Carboxyl esterases (EC 3.1.1.1) and lipases (EC 3.1.1.3) are enzymes that catalyze the cleavage of an ester bond between a carboxylic acid and an alcohol group. The TtEst2 enzyme reveals an open substrate binding site, which is solvent accessible due to the absence of the usual ‘cap’ domain which is present in TtEst.

The purified TtEst2 enzyme has been crystallized and the structures have been determined of both the native enzyme and its complexes with three different reaction products. This information has provided an insight into the substrate specificity of this novel thermophilic carboxyl esterase with respect to its exposed active site and minimal ‘cap’ domain when compared to other members of the α/β hydrolase 3 family.

> AEVGRLRYPPEMPGAEVKVYKKVDNVDLKLYIYKPADWKPADRRSAIVFFFGGGWQSGSPAQFRPQCEYFAGRGMVAMAADYRVGSRHNVKVADCVADAKSAIRWVRQHAAELGVDPQKIVASGGSAGGHLAACTVMVPDLEAPEEDHTISSQANAAILFNPVLILSREGLKDHVPRQDWEERLRERLGTEPKAVSPYHHIRAGLPPMIIFHGTADNTVPFETIRLFAEAMKKAGNRCELVPFEGAAHGFFNFGRGDNLAYQKTLELADEFLVEIGFLAPKGESQP> MRGSHHHHHHGMASMAVSESQL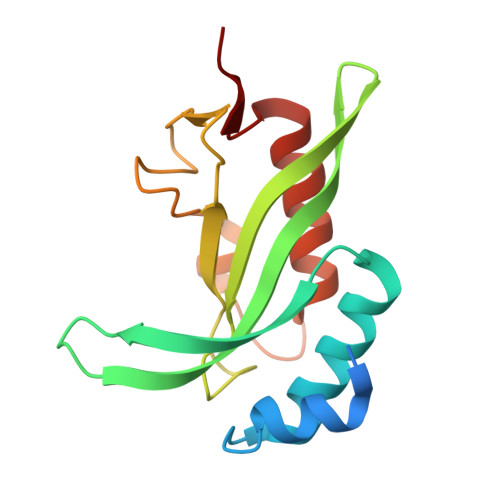KKMVSKYKYRDLTVRETVNVITLYKDLKPVLDSYVFNDGSSRELMNLTGTIPVPYRGNTYNIPICLWLLDTYPYNPPICFVKPTSSMTIKTGKHVDANGKIYLPYLHEWKHPQSDLLGLIQVMIVVFGDEPPVFSRP> MSTIPSEIINWTILNEIISMDDDDSDFSKGLIIQFIDQAQTTFAQMQRQLDGEKNLTELDNLGHFLKGSSAALGLQRIAWVCERIQNLGRKMEHFFPNKTELVNTLSDKSIINGINI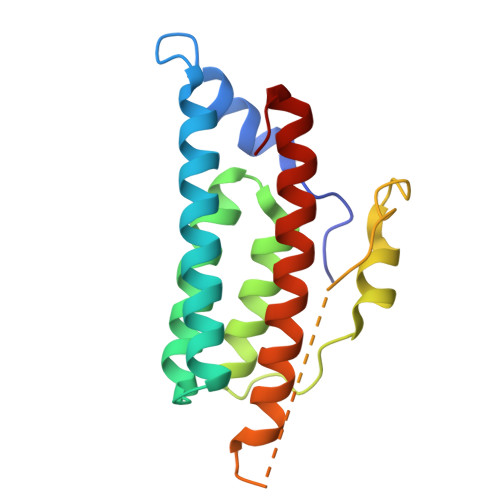DEDDEEIKIQVDDKDENSIYLILIAKALNQSRLEFKLARIELSKYYNTNL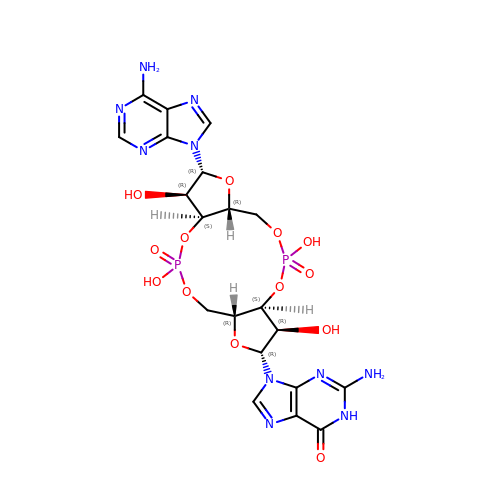2-amino-9-[(2R,3R,3aS,5R,7aR,9R,10R,10aS,12R,14aR)-9-(6-amino-9H-purin-9-yl)-3,5,10,12-tetrahydroxy-5,12-dioxidooctahydro-2H,7H-difuro[3,2-d:3',2'-j][1,3,7,9,2,8]tetraoxadiphosphacyclododecin-2-yl]-1,9-dihydro-6H-purin-6-one | C20 H24 N10 O13 P2 | RFCBNSCSPXMEBK-INFSMZHSSA-N> MRRNILLVQFVGVLLLLPSIMSGQQHSSDNKNWAEKGIVIREVEILGKRPMKDIGVQQTRFDSLVLKENIALSMADILTFNSSIFVKSYGRATLSTVSFRGTSASHTQVTWNGMRINNPMLGMTDFSMIPSYFIDDASLLHGTSSVNMAGGGLGGLVKLSTVPAHQEGFGMQYVQGIGSFSTFDEFLQLKYGDKHWQISTRAVYQSSPNDYKYRNHDKKENIYDDKYNIIEQYYPIERNRSGAYKDLHILQEVYY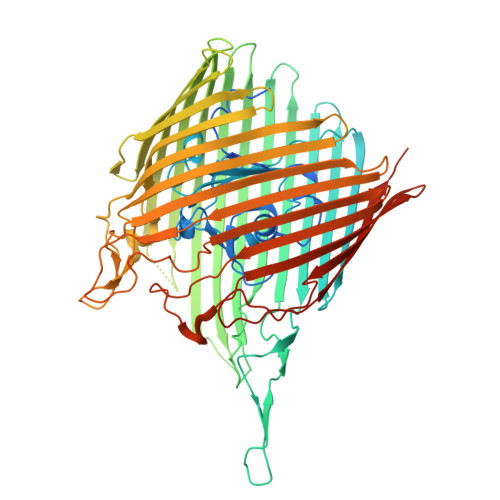NTGKGDRFGLNAWYTDSNRELALLTTDQGDLMDFENRQREHTLRSVLSWDHTRENWKVSARGGYVHTWLAYDYKRDLGNGIMATMTRSRSKVNTFYGQLDGEYFFSDKLLLTAGVSAHQHLVNSLDKDLNKDDNKNDKYGQGRKNDSIVYFDKGRIELSGNVSLKWQPVNRLGMSLVLRGEMFGTKWAPVIPAFFVDYVLSKRGNIMAKASITRNYRFPTLNDLYFLPGGNPALNNESGFTYETGLSFSVDKDNVYTLSGSASWFDQHINDWIIWLPTSKGFYSPVNLKKVHAYGVEVQADYAVAIDKAWKLGLNGTFAWTPSINEGEPTSKADQSVGKQLPYIPEYSATLSGRLTYRSWGLLYKWCYYSERYTMTSNAVSYTGHLPPYLMSNVTLEKGFSLRWADLSLKGTVNNLFDEEYLSVLSRPMPGINFEFFIGITPKWGKKKKGGGHHHHHH> MALAKRIIAALIVKDGRVVKGSNFENLRDSGDPVELGKFYSEIGIDELSFADITASVEKRKTMLELVEKVAEQIDIPFTVGGGIHDFETASELILRGADKVEINTAAVENPSLITQIAQTFGSQAVVVYIAAKRVDGEFMVFTYSGKKNTGILLRDWVVEVEKRGAGEIVLGSIDRLGTKSGYDTEMIRFVRPLTTLPIIAHGGAGKMEHFLEAFLAGADAAKANSVLHFREIDVRELKEYLKKHGVNVRLEGLGSLEHHHHHH

Computational design of KE07 involved construction of a theozyme to catalyze the chemical reaction, which was then grafted into the scaffold of imidazole glycerol phosphate synthase (HisF) from Thermotoga maritima. Catalytically essential residues from the initial design include a base (Glu101) that facilitates C−H bond cleavage, an H-bond donor (Lys222) to stabilize the phenoxide intermediate, and a π-stacking residue (Trp50), which was designed to stabilize the transition state and favor substrate binding through interactions with the aromatic ring of the substrate. This initial KE07 design (Round 1; R1) catalyzes the cleavage of 5-nitrobenzisoxazole, with 103-fold rate acceleration over the noncatalyzed reaction and a turnover rate (kcat) of 0.018 s−1.

Trp50 in the active site of KE07 is a convenient spectroscopic handle to interrogate the active site environment (a second tryptophan residue, Trp156, is invariant throughout evolution). A Trp50Ala mutation was made in KE07 R1 to assess the contribution of Trp50 to the fluorescence; the crystal structures showed no major changes to the active site nor overall fold. This showed that the overall fluorescence of the R1 Trp50Ala mutant was slightly lower than R1, which is consistent with some quenching of the fluorescence of Trp156 by Trp50, similar to what has been reported previously. The Trp50Ala mutants in R1 and R7-2 result in significant (>95%) reductions in kcat, although the KM of R7-2_Trp50Ala increased sevenfold, whereas the KM of R1_Trp50Ala was unchanged, suggesting more involvement of Trp50 in substrate binding in the evolved configuration C.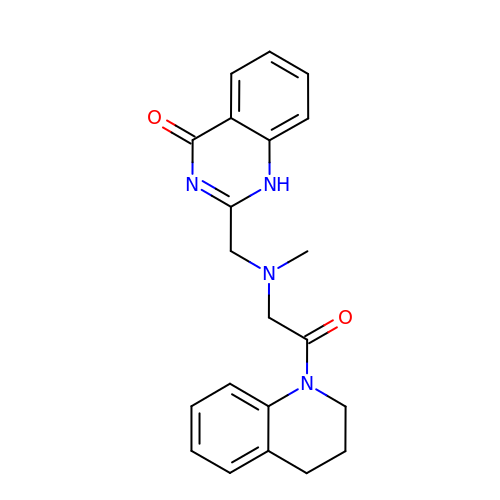2-({[2-(3,4-dihydroquinolin-1(2H)-yl)-2-oxoethyl](methyl)amino}methyl)quinazolin-4(1H)-one | C21 H22 N4 O2 | MTDOUFMMCOQZJF-UHFFFAOYSA-N>[3x]PPGPPGPPGPPGPPAPPGP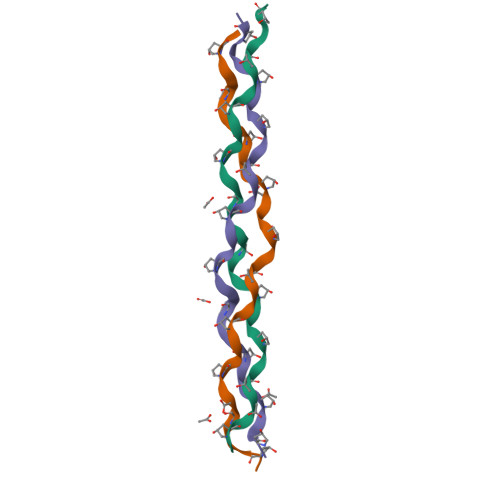PGPPGPPGPPG> TENILRKSDEEIQKEITARVKALESMLIEQGILTTSMIDRMAEIYENEVGPHLGAKVVVKAWTDPEFKKRLLADGTEACKELGIGGLQGEDMMWVENTDEVHHVVVCTLCSCTPWPVLGLPPNWFK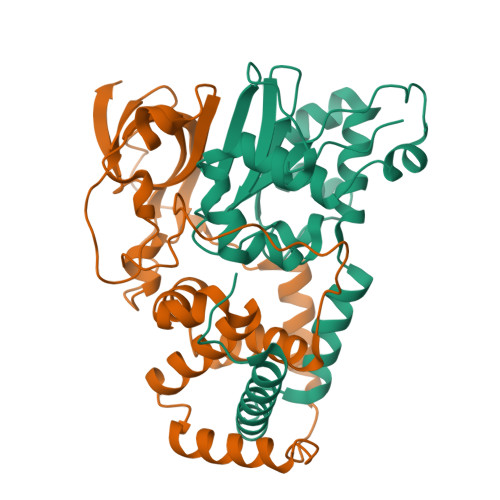EPQYRSRVVREPRQLLKEEFGFEVPPSKEIKVWDSSSEMRFVVLPQRPAGTDGWSEEELATLVTRESMIGVEPAKAV;> MNGVYDVGGTDGLGPINRPADEPVFRAEWEKVAFAMFPATFRAGFMGLDEFRFGIEQMNPAEYLESPYYWHWIRTYIHHGVRTGKIDLEELERRTQYYRENPDAPLPEHEQKPELIEFVNQAVYGGLPASREVDRPPKFKEGDVVRFSTASPKGHARRARYVRGKTGTVVKHHGAYIYPDTAGNGLGECPEHLYTVRFTAQELWGPEGDPNSSVYYDCWEPYIELVDT>ADGNNIKAPIETAVKPPHRTEDNIRDEARRNRSNAVNPFSAKYVPFNAAPGSTESYSLDEIVYRSRSGGLLDVEHDMEALKRFDGAYWRDLFDSRVGKSTWPYGSGVWSKKEWVLPEIDDDDIVSAFEGNSNLFWAERFGKQFLGMNDLWVKHCGISHTGSFKDLGMTVLVSQVNRLRKMKRPVVGVGCASTGDTSAALSAYCASAGIPSIVFLPANKISMAQLVQPIANGAFVLSIDTDFDGCMKLIREITAELPIYLANSLNSLRLEGQKTAAIEILQQFDWQVPDWVIVPGGNLGNIYAFYKGFKMCQELGLVDRIPRMVCAQAANAN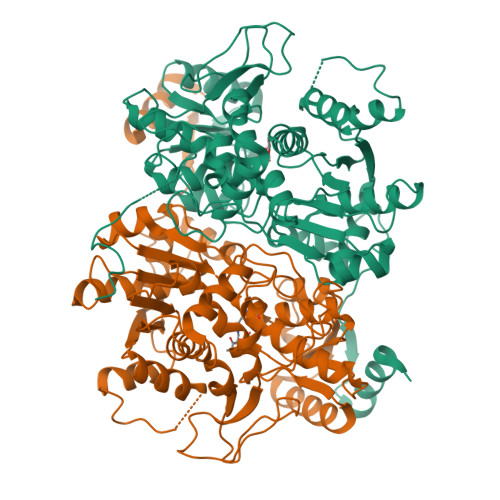PLYLHYKSGWKDFKPMTASTTFASAIQIGDPVSIDRAVYALKKCNGIVEEATEEELMDAMAQADSTGMFICPHTGVALTALFKLRNQGVIAPTDRTVVVSTAHGLKFTQSKIDYHSNAIPDMACRFSNPPVDVKADFGAVMDVLKSYLGSNTLTS[2x]5'-[(1H-BENZIMIDAZOL-2-YLACETYL)AMINO]-5'-DEOXYCYTIDINE 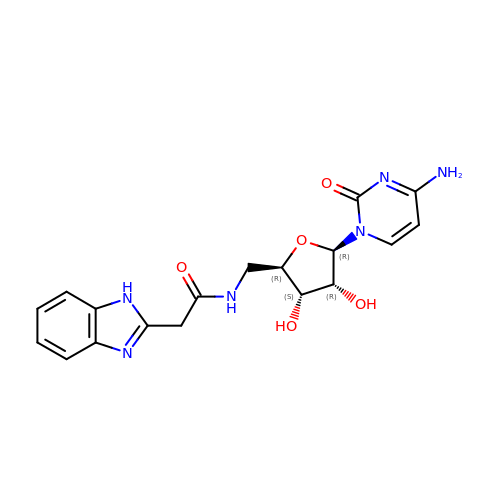| C18 H20 N6 O5 | MMCWRTZSCVUETH-GAEVZRCVSA-N>[2x]SNAMSLLEQLDKNIAASGGLIVSCQPVPGSPLDKPEIVAAMALAAEQAGAVAVRIEGIDNLRMT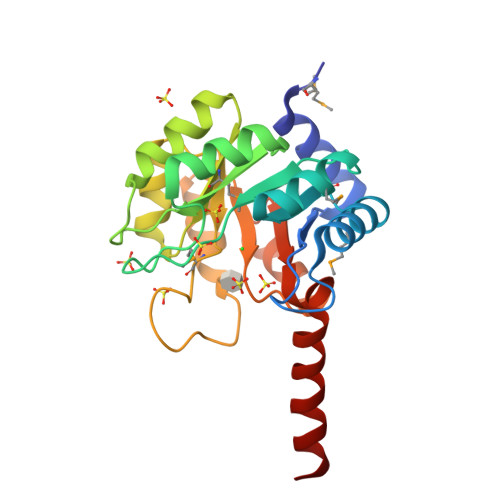RSLVSVPIIGIIKRDLDESPVRITPFLDDVDALAQAGAAIIAVDGTARQRPVAVEALLARIHHHHLLTMADCSSVDDGLACQRLGADIIGTTMSGYTTPDTPEEPDLPLVKALHDAGCRVIAEGRYNSPALAAEAIRYGAWAVTVGSAITRLEHICGWYNDALKKAAS> MAIEQKLMDDHHEVDPR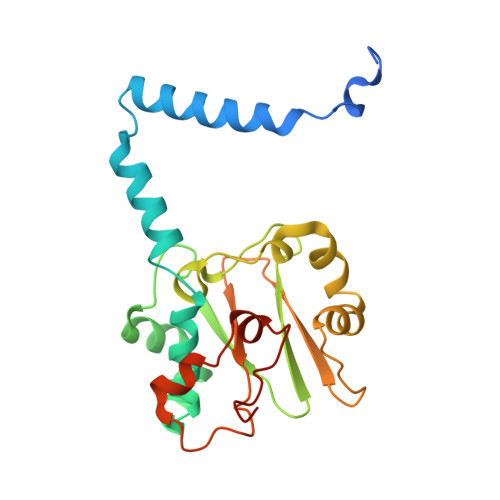FPHHHPRPQSFWEARAKALESLLIEKRLLSSDAIERVIKHYEHELGPMNGAKVVAKAWTDPEFKQRLLEDPETVLRELGYFGLQGEHIRVVENTDTVHNVVVCTLCSCYPWPLLGLPPSWYKEPAYRSRVVKEPRKVLQEFGLDLPDSVEIRVWDSSSEVRFMVLPQRPEGTEGMTEEELAQIVTRDSMIGVAKVQPPKVIQE>MDIKINDITLGNNSPFVLFGGINVLESLDSTLQTCAHYVEVTRKLGIPYIFKASFDKANRSSIHSYRGVGLEEGLKIFEKVKAEFGIPVITDVHEPHQCQPVAEVCDVIQLPARLAQQTDLVVAMAKTGNVVNIKKPQFLSPSQMKNIVEKFHEAGNGKLILCERGSSFGYDNLVVDMLGFGVMKQTCGNLPVIFDVTHSLQTRDAGSAASGGRRAQALDLALAGMATRLAGLFLESHPDPKLAKCDGPSALPLHLLEDFLIRIKAL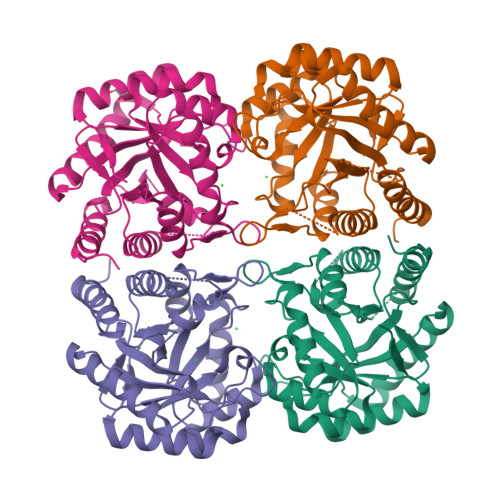DDLIKSQPILTIE[4x]>MSKTQEFRPLTLPPKLSLSDFNEFIQDIIRIVGSENVEVISSKDQIVDGSYMKPTHTHDPHHVMDQDYFLASAIVAPRNVADVQSIVGLANKFSFPLWPISIGRNSGYGGAAPRVSGSVVLDMGKNMNRVLEVNVEGAYCVVEPGVT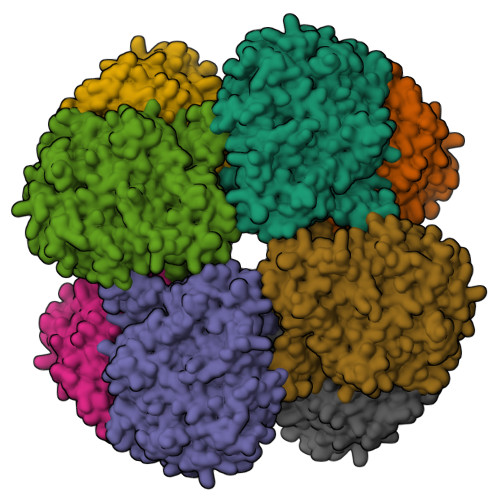YHDLHNYLEANNLRDKLWLDVPDLGGGSVLGNAVERGVGYTPYGDHWMMHSGMEVVLANGELLRTGMGALPDPKRPETMGLKPEDQPWSKIAHLFPYGFGPYIDGLFSQSNMGIVTKIGIWLMPNPRGYQSYLITLPKDGDLKQAVDIIRPLRLGMALQNVPTIRHILLDAAVLGDKRSYSSRTEPLSDEELDKIAKQLNLGRWNFYGALYGPEPIRRVLWETIKDAFSAIPGVKFYFPEDTPENSVLRVRDKTMQGIPTYDELKWIDWLPNGAHLFFSPIAKVSGEDAMMQYAVTKKRCQEAGLDFIGTFTVGMREMHHIVCIVFNKKDLIQKRKVQWLMRTLIDDCAANGWGEYRTHLAFMDQIMETYNWNNSSFLRFNEVLKNAVDPNGIIAPGKSGVWPSQYSHVTWKL[2x]(3R)-1-{[1-(5-fluoro-2-{[4-(2-hydroxyethoxy)-3,5-dimethylphenyl]amino}pyrimidin-4-yl)-4-methyl-1H-pyrrol-3-yl]methyl}pyrrolidin-3-ol 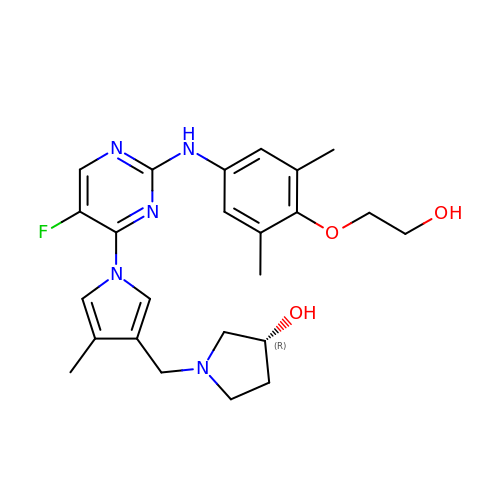| C24 H30 F N5 O3 | OSONANZITXBMIW-HXUWFJFHSA-N> GSFVEMVDNLRGKSGQGYYVEMTVGSPPQTLNILVDTGSSNFAVGAAPHPFLHRYYQRQLSSTYRDLRKGVYVPYTQGKWEGELGTDLVSIPHGPNVTVRANIAAITESDKFFINGSNWEGILGLAYAEIARPD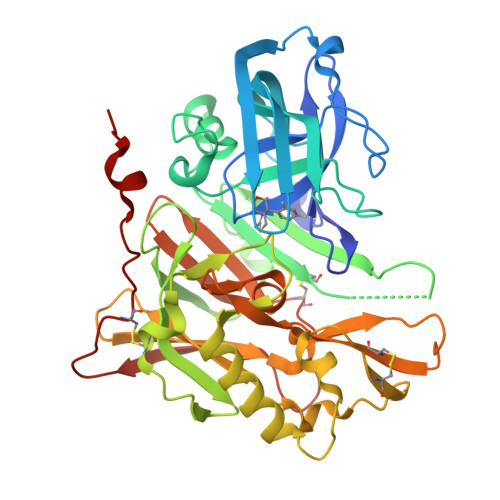DSLEPFFDSLVKQTHVPNLFSLQLCGAGFPLNQSEVLASVGGSMIIGGIDHSLYTGSLWYTPIRREWYYEVIIVRVEINGQDLKMDCKEYNYDKSIVDSGTTNLRLPKKVFEAAVKSIKAASSTEKFPDGFWLGEQLVCWQAGTTPWNIFPVISLYLMGEVTNQSFRITILPQQYLRPVEDVATSQDDCYKFAISQSSTGTVMGAVIMEGFYVVFDRARKRIGFAVSACHVHDEFRTAAVEGPFVTLDMEDCGYNIPQTDESRSHHHHHH>MAKKTSSGSETPDLTVATRTGSKDLPIRNIPGNYGLPIVGPIKDRWDYFYDQGAEEFFKSRIRKYNSTVYRVNMPPGAFIAENPQVVALLDGKSFPVLFDVDKVEKKDLFTGTYMPSTELTGGYRILSYLDPSEPKHEKLKNLLFFLLKSSRNRIFPEFQATYSELFDSLEKELSLKGKADFGGSSDGTAFNFLARAFYGTNPADTKLKADAPGLITKWVLFNLHPLLSIGLPRVIEEPLIHTFSLPPALVKSDYQRLYEFFLESAGEILVEADKLGISREEATH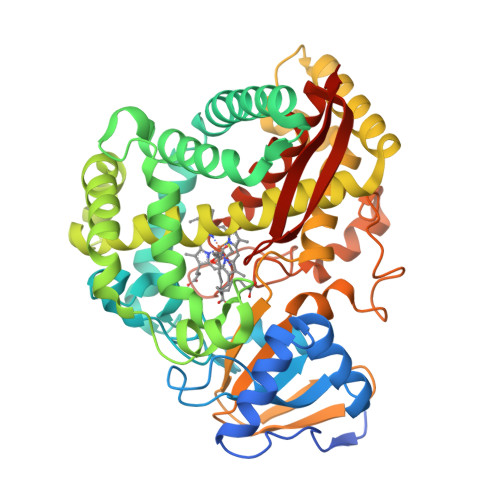NLLFATCFNTWGGMKILFPNMVKRIGRAGHQVHNRLAEEIRSVIKSNGGELTMGAIEKMELTKSVVYECLRFEPPVTAQYGRAKKDLVIESHDAAFKVKAGEMLYGYQPLATRDPKIFDRADEFVPERFVGEEGEKLLRHVLWSNGPETETPTVGNKQCAGKDFVVLVARLFVIEIFRRYDSFDIEVGTSPLGSSVNFSSLRKASFHHHH[2x]>MIERLVTLCFNRRGIVALVFAMVALYGWYAWKQLPLEAYPDIADTTSQVVTQVNGLAAEEVEQQITIPLEREIMGVPGMHVMRSKSTFGLSLITVVFKDGAEDYWSRQRLQERINGVSLPYGAQPSLDPLTSPIGEIYRYTLVSKTRDLRELSELQFWKVIPRLKQVAGVVDVANFGGLTTQFMLEFDPVMLSKYNISLNQITQAISENNANAGGSILNRGEQGLVVRGVGLIRNLDDLGNIVVTQKNGVPVLVKDLGRVVLGNPQRHGILGMDRNPDTIQGITLLLKNENPSVVMEGVHAAVRDLNDNILPKDVKVVPYIDRSNLVDATVHTVGKTLMEGMFLVSLVLLLFLGSPRAAIIVAVTIPLSLLMAFILMHHFKIPANLLSLGAIDFGIIVDGAIVVMENILRRREEDAEKELHGRDIMQSVL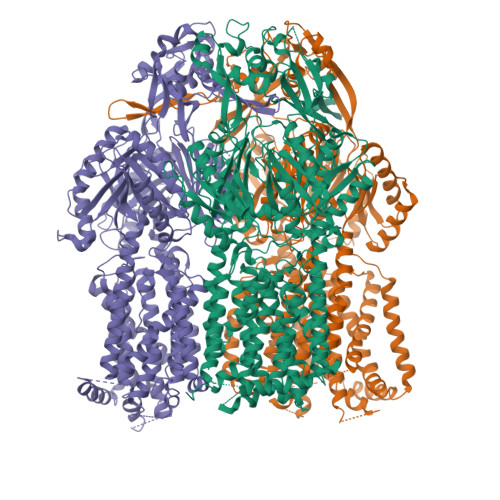QVARPIFFGMIVIITAYLPLFAFQRIEYKLFSPMAFAVGFALFGALLVALLLIPGLAYWAYRKPRKVFHNPALVWLAPRYESVLNRLVGSTRTAIGIAVATLVGVMILGATIGRDFLPYLDEGSIWLQVTLPPGISLEKAGQMADNLRAATMEFPEVEHVVTQVGRNDEGTDPFSPSHIETAVTLHPYSTWTSGRDKQQLIEAMATRFRDLPGTQVGFSQPMIDGVLDKLAGAHSDLVVKVYGNDFAETRQVATAITRLLKTVPGAQDVIIDQEPPLPQVRIDVDRAAAARLGINVADVMALIQTGIGGSPVTQVFVEDRSYNVVARFIGSSRNDPEAIGNLTLTAANGAHVALAQVAHIRLAEGETTITREMNKRHLTVRLNLRGRDLSTFLEEARMRIDKEVPYDRTHIQVAWGGQFENQQRAQARLAVILPMVLALMFVLLFGEFKNLRQPALILMAVPLATLGGLVALHLRGMTLNVSSAVGFIALFGVAVLNAIIMIANLNRWRDTSGVSLKEAVVRGAGERMRPVLMTATVAALGLIPAALAHGLGSDVQRPLATVVVGGLITATALTLVLLPALYYLIETRAAKQVREEPPVQFGPTSEGDLHHHHHH[6x]>FSSREQPQQNECQIQKLNALKPDNRIESEGGLIETWNPNNKPFQCAGVALSRCTLNRNALRRPSYTNGPQEIYIQQGKGIFGMIYPGCPSTFEEPQQPQQRGQSSRPQDRHQKIYNFREGDLIAVPTGVAWWMYNNEDTPVVAVSIIDTNSLENQLDQMPRRFYLAGNQEQEFLKYQQEQGGHQSQKGKHQQEEENEGGSILSGFTLEFLEHAFSVDKQIAKNLQGENEGEDKGAIVTVKGGLSVIKPPTDEQQQRPQEEEEEEEDEKPQCKGKDKHCQRPRGSQSKSRRNGIDETICTMRLRHNIGQTSSPDIYNPQAGSVTTATSLDFPALSW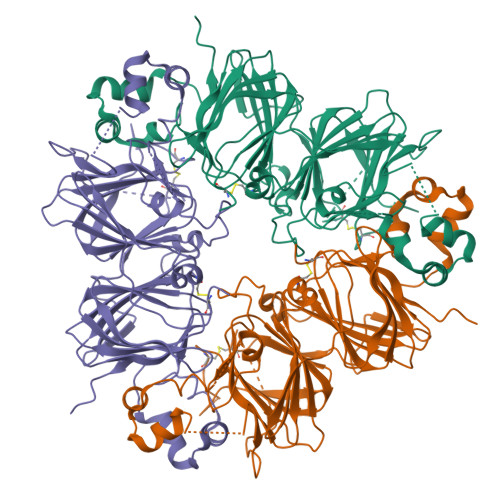LRLSAEFGSLRKNAMFVPHYNLNANSIIYALNGRALIQVVNCNGERVFDGELQEGRVLIVPQNFVVAARSQSDNFEYVSFKTNDTPMIGTLAGANSLLNALPEEVIQHTFNLKSQQARQIKNNNPFKFLVPPQESQKRAVA[3x]N-[4-fluoro-5-({(2S,4S)-2-methyl-4-[(5-methyl-1,2,4-oxadiazol-3-yl)methoxy]piperidin-1-yl}methyl)-1,3-thiazol-2-yl]acetamide | C16 H22 F N5 O3 S | 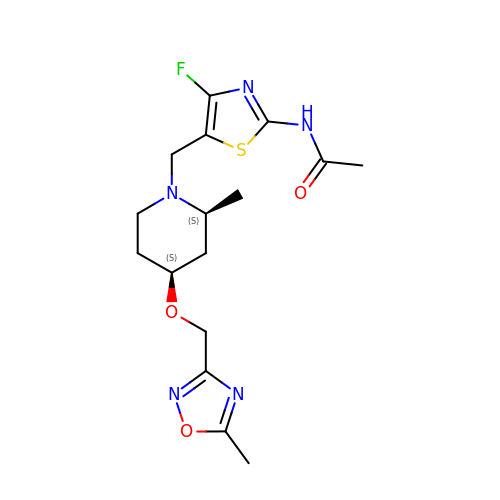FRVXHWNHGWUTQO-CABZTGNLSA-N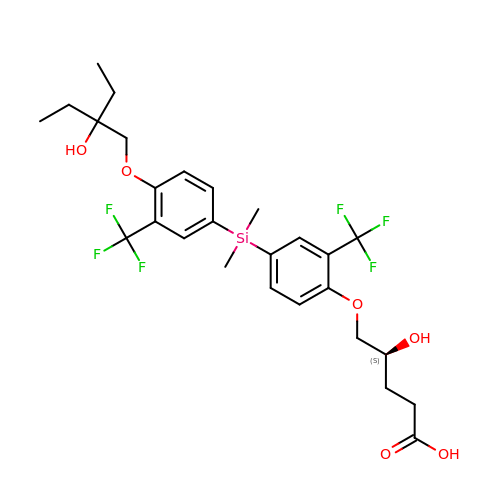(4~{S})-5-[4-[[4-(2-ethyl-2-oxidanyl-butoxy)-3-(trifluoromethyl)phenyl]-dimethyl-silyl]-2-(trifluoromethyl)phenoxy]-4-oxidanyl-pentanoic acid | C27 H34 F6 O6 Si | FOBWZYOIZWJMHE-QGZVFWFLSA-N> HHHHHHSKEELLKLTETVVTEYLNSGNANEAVNGVREMRAPKHFLPEMLSKVIILSLDRSDEDKEKASSLISLLKQEGIATSDNFMQAFLNVLDQCPKLEVDIPLVKSYLAQFAARAIISELVSISELAQPLESGTHFPLFLLCLQQLAKLQDREWLTELFQQSKVNMQKMLPEIDQNKDRMLEILEGKGLSFLFPLLKLEKELLKQIKLDPSPQTIYKWIKDNISPKLHVDKGFVNILMTSFLQYISSEVNPPSDETDSSSAPSKEQLEQEKQL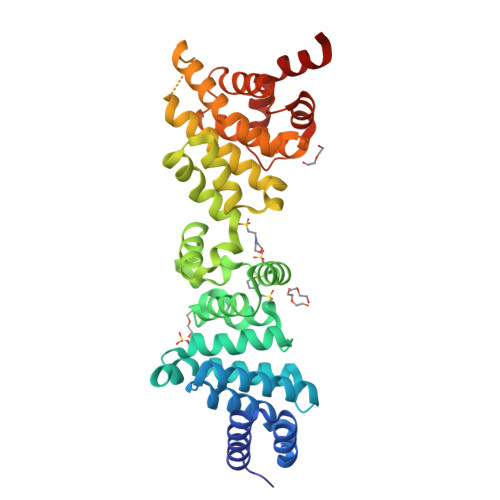LLSFKPVMQKFLHDHVDLQVSALYALQVHCYNSNFPKGMLLRFFVHFYDMEIIEEEAFLAWKEDITQEFPGKGKALFQVNQWLTWLETA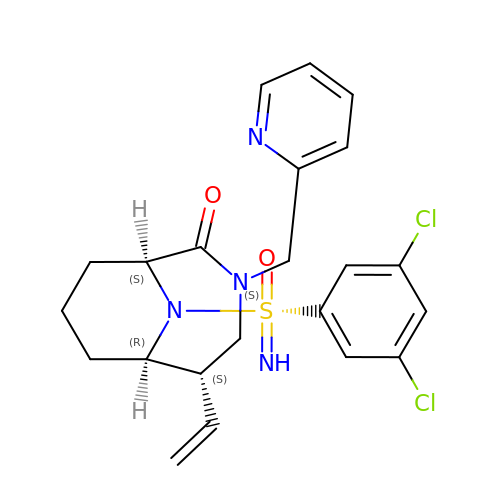(1S,5S,6R)-10-[[3,5-bis(chloranyl)phenyl]sulfonimidoyl]-5-ethenyl-3-(pyridin-2-ylmethyl)-3,10-diazabicyclo[4.3.1]decan-2-one | C22 H24 Cl2 N4 O2 S | CQIWVXGAJXNGRQ-BJHMJODQSA-N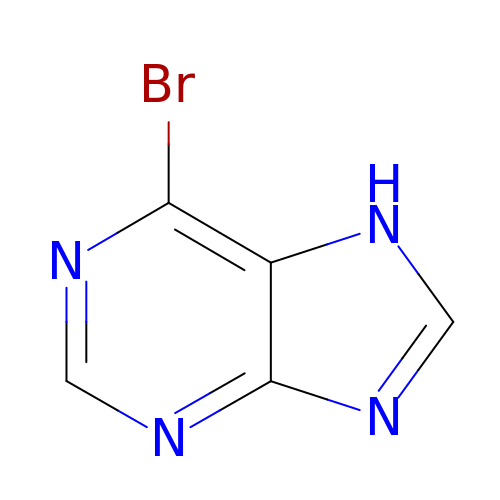6-BROMO-7H-PURINE | C5 H3 Br N4 | CTGFGRDVWBZYNB-UHFFFAOYSA-N> PISPIETVPVKLKPGMDGPKVKQWPLTEEKIKALVEICTEMEKEGKISKIGPENPYNTPVFAIKKKDSTKWRKLVDFRELNKRTQDFWEVQLGIPHPAGLKKKKSVTVLDVGDAYFSVPLDEDFRKYTAFTIPSINNETPGIRYQYNVLPQGWKGSPAIFQSSMTKILEPFRKQNPDIVIYQYMDDLYVGSDLEIGQHRTKIEELRQHL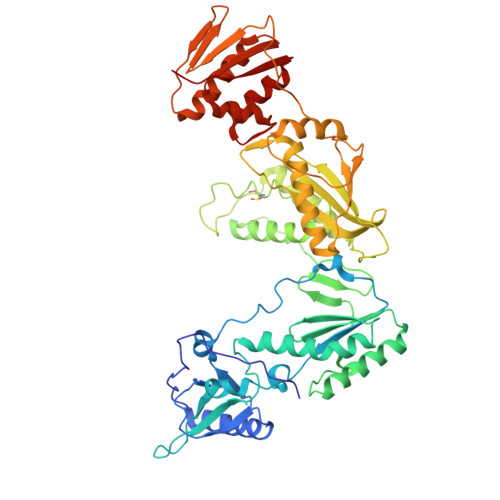LRWGLTTPDKKHQKEPPFLWMGYELHPDKWTVQPIVLPEKDSWTVNDIQKLVGKLNWASQIYPGIKVRQLCKLLRGTKALTEVIPLTEEAELELAENREILKEPVHGVYYDPSKDLIAEIQKQGQGQWTYQIYQEPFKNLKTGKYARMRGAHTNDVKQLTEAVQKITTESIVIWGKTPKFKLPIQKETWETWWTEYWQATWIPEWEFVNTPPLVKLWYQLEKEPIVGAETFYVDGAANRETKLGKAGYVTNRGRQKVVTLTDTTNQKTELQAIYLALQDSGLEVNIVTDSQYALGIIQAQPDQSESELVNQIIEQLIKKEKVYLAWVPAHKGIG> MSEFRIHHDVNELLSLLRVHGGDGAEVYIDLLQKNRTPYVTTTVSAHSAKVKIAEFSRTPEDFLKKYDELKSKNTRNLDPLVYLLSKLMEDRETLQYLQQNAKERAELAASAAASSTASFGASATASKISMQELEELRKQLGSVATGPTWQQSLELTRKMLRDKQSKKNSGQRLPVLPAWVYERPALLGDFLPGTGGSADTAVPIGSLPLASQEAAVVEDLLYVLVGVDGRYISAQPLTGRQGRTFLVDPNLDLSIRELVSRILPVAASYSTVTRFIEEKSSFEYGQVNHALAAAMRTLVKEYLVLVTQLEQLQRQGLLSLQKLWFYIQPAMRSLDILASLATSVDKGECIGGATLSLLHDRSFSYTGDSQAQELCLHLTKAASTPYFEILEKWIYRGIIDDPYSEFMVEEHELRKEKIQEDYNDKYWDQRYTVVQRQIPSFLQKMAGKVLSTGKYLNVVRECGHDVTCPVAKEVVYTLKERAYVEQIEKAFSYASKVLLDFLMGEKELLAHLRSIKRYFLMDQGDFFVHFMDLTEEELKKPVDDITPTRLEALLELALRMSTANTDPFKDDLKIDLMPHDLITQLLRVLAIETQQEKAMVHADPTELTLSGLEAFSFDYVVTWPLSLIINRKALTRYQMLFRHMFYCKHVERQLCSVWISNKAAKRFSLHSAKWFAGAFTLRQRMLNFVQNIQSYMMFEVMEPTWHVLEQNLRSASNIDDVLGHHASFLDNCLKDCMLTNPELLRVFSKLMSVCVMFTNCLQRFTQSMKLDSELGHPALEPGAMLGPPTEAERAEERARKELARKCLAEHVDAPQLASSFEATITKFDKNFSAHLLDLLARLSIYSTSDCEHGMASVISRLDFNGFYTERLERLSAERSQKAAPPVPGPRGPPALVPRVAVTAQ;> MATPDQKSPNVLLQNLCCRILGKSEADVAQQFQYAVRVIGSNFAPTVERDEFLVAEKIKKELTRQRREADAALFSELHRKLHSQGVLKNKWSILYLLLSLSEDPRKQPSKVSGYAALFAQALPRDAH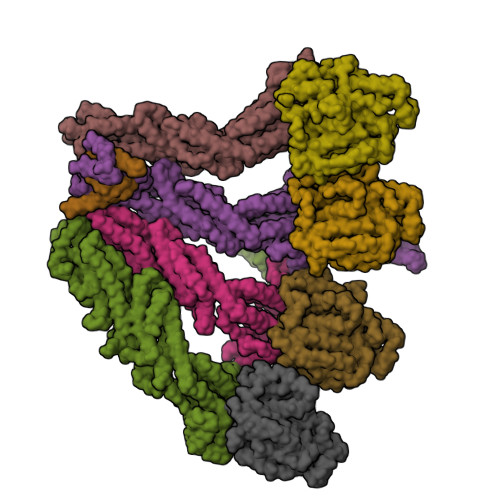STPYYYARPQSLPLNYQERGAPSAQSAGSAGSSGVSSLGTYALNGPTPPPPPPALLPGQPLPAPGVGDGLRQQLGSRLAWTLTASQPSLPSTTSKAVPSSGSRGAARPRREGDAAAGAVEVTEAALVRDILYVFQGIDGKHVKMSNADNCYTVEGKANLSKSLRDTAVRLAELGWLHNKIRKYTDQRSLDRSFGLVGQSFCAALHQELREYYRLLSVLHSQLQLEDDQGVNLGLESSLTLRRLLVWTYDPKMRLKTLAALVDHCQGRKGGELASAVHAYTKTGDPYARSLVQHILSLVSHPVLSFLYRWIYDGELEDTYHEFFVASDPAVKADRLWHDKYALRKPMIPSFMTMDQCRKVLLIGKSINFLHQVCHDQTPTTKMIAVTKSAESPQDAADLFTDLENAFQGKIDAAYFETSKYLLDVLNKKYSLLDHMQAMRRYLLLGQGDFIRHLMDLLKPELVRPATTLYQHNLTGILETAVRATNAQFDSPEILKRLDVRLLEVSPGDTGWDVFSLDYHVDGPIATVFTRECMSHYLRAFNFLWRAKRVEYILTDIRKGHMCNARLLRSMPEFSGVLHHCHILASEMVHFIHQMQYYVTFEVLECSWDELWNRVQRAQDLDHIIAAHEAFLGTVISRCLLDSDSRALLNQLRAVFDQIIELQNTQDAIYRAALEELQRRLQFEEKKKQREAEGQWGVSAAEEEQEKRRVQEFQESIPKMCSQLRILTHFYQGVVQQFLVSLTTSSDESLRFLSFRLDFNEHYRAREPRLRVSLGTRGRRSSHT;> MIHELLLALSGYPGSIFTWNKRGGLQVSQDFPFLHPSETSVLNRLCRLGTDYIRFTEFIEQYTGHVQQQDHHPSQQGQGGLHGIYLRAFCTGLDSVLQPYRQALLDLEQEFLADPHLSISHINYSLDQFQLLFPSVMVVVEQIKSQKIHGCQILETVYKHSCGGLPPVRSALEKILAVCHGVMYKQLSAWMLHGLLLDQHEEFFIKQGPSSGNVSAQPEEDEEDLGIGGLTGKQLRELQDLRLIEEENMLAPSLKQFSLRVEILPSYIPVRVAEKILFVGESVQMFENQNVNLTRKGSILKDQEDTFAAELHRLKQQPLFSLVDFEQVVDRIRSTVAEHLWKLMVEESDLLGQLKIIKDFYLLGRGELFQAFIDTAQHMLKTPPTAVTEHDVNVAFQQSAHKVLLDDDNLLPLLHLTIEYHGKEHKADATQAREGPSRETSPREAPASGWAALGLSYKVQWPLHILFTPAVLEKYNVVFKYLLSVRRVQAELQHCWALQMQRKHLKSNQTDAVKWRLRNHMAFLVDNLQYYLQVDVLESQFSQLLHQINSTRDFESIRLAHDHFLSNLLAQSFILLKPVFHCLNEILDLCHSFCSLVSQNLGPLDERGAAQLSILVKGFSRQSSLLFKILSSVRNHQINSDLAQLLLRLDYNKYYTQAGGTLGSFGM;> MASPAPSWTRLDPQQERDVRELIRLVSGVQDEADPNFQLALHFAWSNFRFHRFLDVNSHKVEKTIEGIYEKFIIHSDLSKAASWKRLTDEFLNASLPSIKEIKTDAHYSILSLLLCLSDSPSNSNYVETPRNKEVEKKDDFDWGKYLMEGEEIDLGPNVDTPNWSEESEDEDDPQPLSREDSGIQVDRTPLEEQDQSRKPASRVSWKVDEPDARSWLEQHVVRQYWTTRSSKFPHSLHLHSNLAAVWDQHLYSSDPLYVPDDRVSVTETQVIRETLWLLSGVKKLFIFQLIDGKVAVRNNIMVTHLTHSCLRSVLEQIAAYGQVVFRLQEFIDEVMGHSSESTLPGNGSVPKKSTDAPFRTYQAFMWALYKYFISFKEELSEIEKCIINNDTTVTLAIVVDKLSPRLAQLKVLHKVFSTGVAEVPPDTRNVVRASHLLNTLYKAILEYDNVGEASEQTVSLLFSLWVETVRPYLQIVDEWIVHGHLCDGAREFIIQRNKNVPVNHRDFWYATYTLYSVSEKTENEEKMSDNASASSGSDQGPSSRQHTMVSFLKPVLKQIIMAGKSMQLLKNLQCAESTTCQAMARDAERKSLYTLFLESVQSRLRHGEDATAQALTEQQATRETLIKMQSIAERHLELDDVHDPLLAINFARLYLEQSDFHEKFAGGDICVDRSSESVTCQTFELTLRSCLYPHIDKQYLDCCGNLMRTLKKDYRLVEYLQAMRNFFLMEGGDTMYDFYTSIFDKIREKETWQNVSFLNVQLQEAVGQRYPEDSSRLSISFENTDTAKKKLPVHTLDGLTLSYKVPWPVDIVISLECQKIYNQVFLLLLQIKWAKYSLDVLLFGELASSAEKPQSKEGLLSGQDTAAQFGPQKEPVRQQIHRMFLLRVKLMHFVNSLHNYIMTRILHSTGLEFQHQVEEAKDLDQLIKIHYRYLSTIHDRCLLREKVSFVKEAIMKVLNLALMFADGWQAGLGAWQMESIEKMESDFKNCHMFLVTILNKAVCRGSFPHLESLALSLMAGMEQKREDDLFNHTWGQGDLPNYTCAVRLLGVRKGGGTRPK;>[2x]MAGNSGSGAAAAANLNAVRETMDVLLEISRILNTGLDMETLSICVRLCEQGINPEALSSVIKELRKATEALKAAENMTS;>[4x]MPREIITLQLGQCGNQIGFEFWKQLCAEHGISPEGIVEEFATEGTDRKDVFFYQADDEHYIPRAVLLDLEPRVIHSILNSPYAKLYNPENIYLSEHGGGAGNNWASGFSQGEKIHEDIFDIIDREADGSDSLEGFVLCHSIAGGTGSGLGSYLLERLNDRYPKKLVQTYSVFPNQDEMSDVVVQPYNSLLTLKRLTQNADCVVVLDNTALNRIATDRLHIQNPSFSQINQLVSTIMSASTTTLRYPGYMNNDLIGLIASLIPTPRLHFLMTGYTPLTTDQSVASVRKTTVLDVMRRLLQPKNVMVSTGRDRQTNHCYIAILNIIQGEVDPTQVHKSLQRIRERKLANFIPWGPASIQVALSRKSPYLPSAHRVSGLMMANHTSISSLFESSCQQYDKLRKREAFLEQFRKEDIFKENFDELDRSREVVQELIDEYHAATRPDYISWGTQEQ>[2x]KGTFKDYVRDRADLN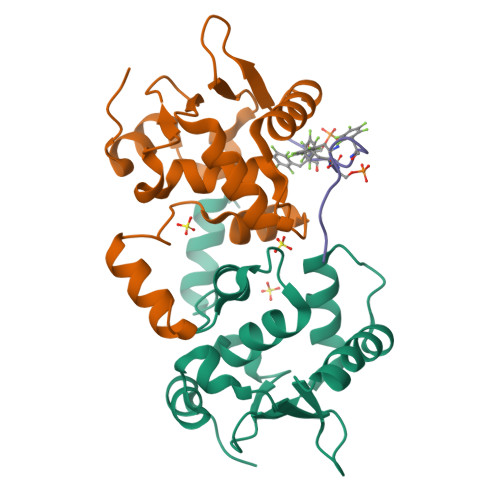KDKPVIPAAALAGYTGSGPIQLWQFLLELLTDKSCQSFISWTGDGWEFKLSDPDEVARRWGKRKNKPKMNYEKLSRGLRYYYDKNIIHKTAGKRYVYRFVCDLQSLLGYTPEELHAMLDVKPDAD;> PSFDSFDFEDFPAALWX>[3x]MAHHHHHHDDDDKIRTLPGEGTQVHPRAPLLQILKVAGAQEEVFTVKEVMHYLGQYIMMKQLYDKQRQHIVHCHDDPLGEL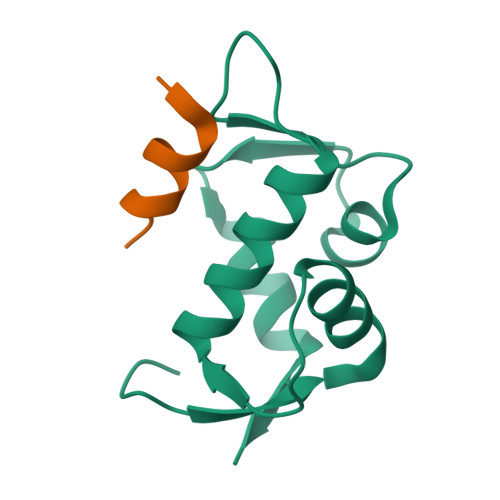LEVGSFSVKNPSPLYEMLKRNLVILNNSDAAKNLSVGKDSNESPSEDPGQVSSGSINSA;>SQETFSDLWKLLPEN[3x]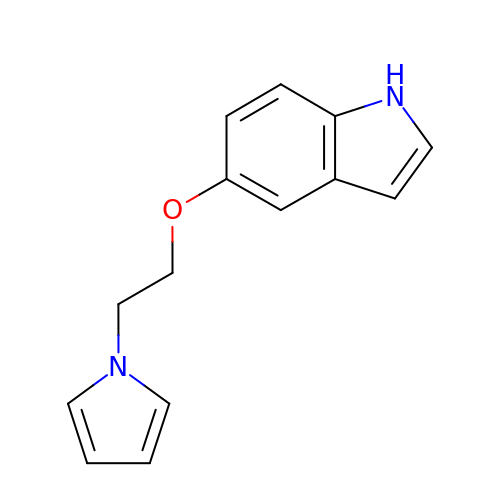5-[2-(1H-pyrrol-1-yl)ethoxy]-1H-indole | C14 H14 N2 O | NSZDJRLPCLOQAM-UHFFFAOYSA-N> MIRNVKKQRPVNLDLQTIRFPITAIASILHRVSGVITFVAVGILLWLLGTSLSSPEGFEQASAIMGSFFVKFIMWGILTALAYHVVVGIRHMMMDFGYLEE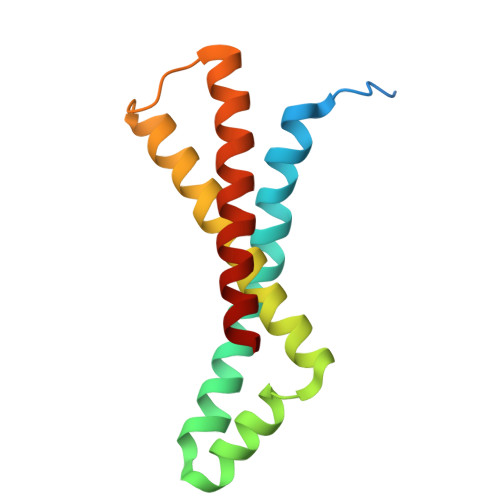TFEAGKRSAKISFVITVVLSLLAGVLVW>[2x]AMITEKSAALYARAVEVMPGGNSRTAVYSSPYPVYVRSGSGARVTDVDGVERIDFLNNSTTLIHGHAHPEMVEAIAAAVGHGTSFGMPTPVEVEYAEALSARNETFEHVRFTSSGTEAVMMAVQAARAYTE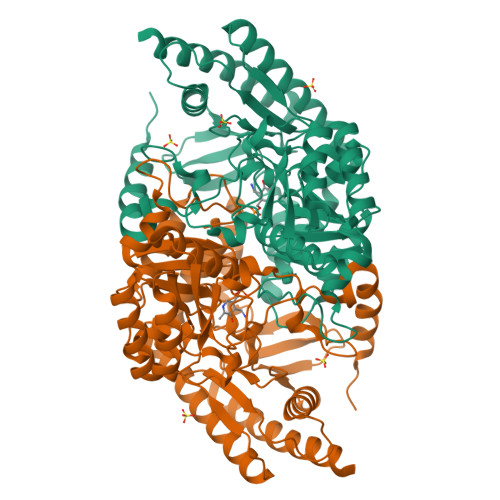RPKIAKIAGAYHGAYDAVAVNNDGSGNLISHAVTGNPEGVVANTVVIPFNDPEGSLEVLRRHADDLACVLIDPVPWRIGLLPASKEWLDALREFCDASGAVLISDEVGSYRVGYHGAMQLLGAEADITVMGKVIAAGMPIGAVAGRRRFMSVFDPSKGKPALPHSGSYNANPVSMSSGIASLRLLTPQAHERIGQLGEQARGSMRTALGEAGLDWEVNGLGSLFRVVANSAPAGYDSAAAAMKALYWKLLENGIHIGDSGLGCISTPMGEEEIAEYAVAFAKSLGQVLAEGRA> GPAGSMATERDQEIIDFIDQGNYTYAQSLITKKLAKSPQKLFYHVLQNEIHLKSGQRELAIKKNLELLNRYPNDPLTIEKLSDFFSKMEMEKESSLVYENAIKKYPVSTETLCLSWFDNSIEKYDFKVFNRIFMYLNKNGKSRLHTLWYAFSFHLLLQEGETDKASLYNSLGKKLMEGLQPFENTQEIYVYTLFLSSKEIEQVLSGVTLPLDLELKLLYMKAMKENASFEALHAYTEKLLFKEKFDDFDTWKLWILSGKEIGKSFEELDQKLTLPTRNISLLKIELDILYSRNIETSVENYYQKFNTKLCCYADLSQYELPTSFIGSLKNSTSEENLITVVNNRKFVNQTDNWDVYERFSTKEGAEYDSNPVNELTLR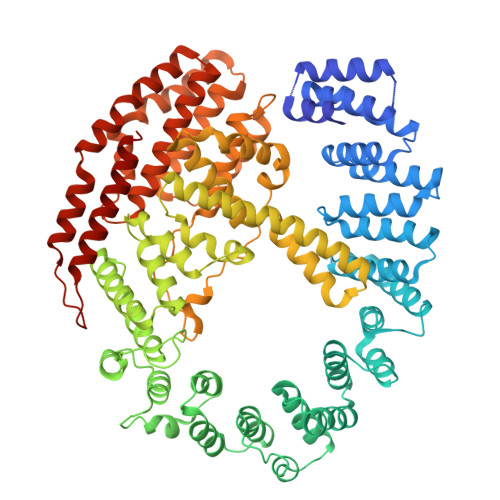TIVSDLDSSPQNTIKNIVLLKHLLEQDKYNYKLKLWLMKLYSQLNTNDLIFPIYNGLKIRMTQHETLNYYLTTTNPSKINLDAWVDIYRFYLTSKQEIKESIIQGFDNGVFNKLEGFINFSKRMQNSISLNFTVAKILQISTILGTDGYLNYFIHYLKTNEALIVSDYTDNRDFKSEWNGLEKIDCIDVPVNDVATKLKLLVYSIVFEDQDASRLLKVFNKITSNAKFSVFDNLLYKLYFNLLKITKTKLNPQETQSLYNYLQKNLKTDKLKILIPENLLSGELTQNLTNLVEFIKIVKLLAKRHPSSYMNQLVNLVKPFGKEFKNLKLVQRQHEIIDSMDFEPPISVDISQTKLEIKSSIEDCVVALLNSL>[2x]MGSRNIVRAVLEEKKTEAITEVDEKGITCVMKFGGSSVASAERMKEVADLILTFPEESPVIVLSAMGKTTNNLLLAGEKAVSCGVSNASEIEELSIIKELHIRTVKELNIDPSVILTYLEELEQLLKGIAMMKELTLRTRDYLVSFGECLSTRIFAAYLNTIGVKARQYDAFEIGFITTDDFTNGDILEATYPAVAKRLYDDWMHDPAVPIVTGFLGKGWKTGAVTTLGRGGSDLTATTIGKALGLKEIQVWKDVDGVLTCDPTIYKRATPVPYLTFDEAAELAYFGAQVLHPQSMRPAREGEIPVRVKNSYNPKAPGTIITKTRDMTKSILTSIVLKRNVTMLDIASTRMLGQVGFLAKVFSIFEEL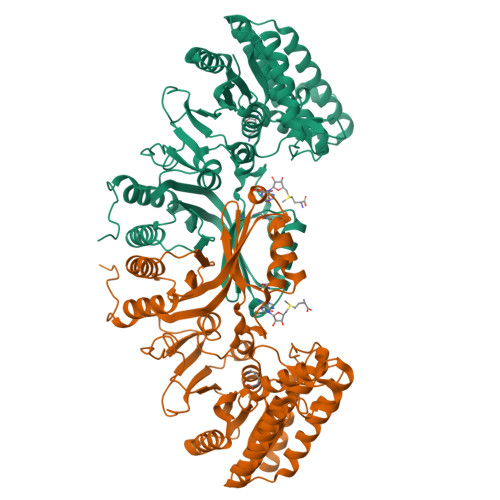GISVDVVATSEVSISLTLDPSKLWSRELIQQELDHVVEELEKIAVVNLLKGRAIISLIGNVQHSSLILERAFHVLYTKGVNVQMISQGASKVNISFIVNEAEAEGCVQALHKSFFESGDLSELLIQPRLGNGSPVRTLQVEN> MKTIFSGIQPSGVITIGNYIGALRQFVELQHEYNCYFCIVDQHAITVWQDPHELRQNIRRLAALYLAVGIDPTQATLFIQSEVPAHAQAAWMLQCIVYIGELERMTQFKEKSAGKEAVSAGLLTYPPLMAADILLYNTDIVPVGEDQKQHIELTRDLAERFNKRYGELFTIPEARIPKVGARIMSLVDPTKKMSKSDPNPKAYITLLDDAKTIEKKIKSAVTDSEGTIRYDKEAKPGISNLLNIYSTLSGQSIEELERQYEGKGYGVF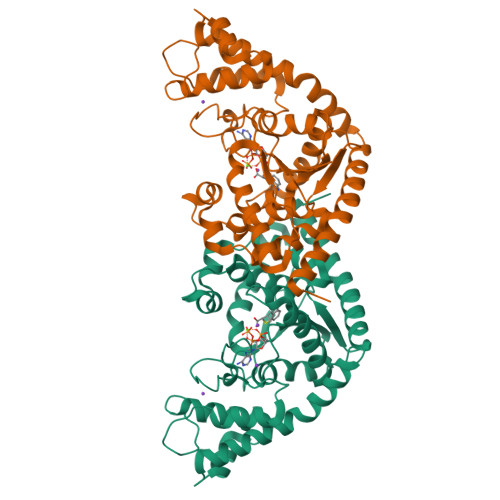KADLAQVVIETLRPIQERYHHWMESEELDRVLDEGAEKANRVASEMVRKMEQAMGLGRRRLE Here we describe a new mechanism by which foot-and-mouth disease virus (FMDV) can become resistant to ribavirin. Amino acid changes in the viral polymerase, selected by ribavirin, are able to modify the types of mutations produced in the presence of ribavirin. P44S but not P169S was detected in a 70% proportion in R-Ap35, as evidenced by analysis of both the consensus sequences and their corresponding mutant spectra. These results suggest that the three substitutions in 3D were selected sequentially during replication in the presence of increasing concentrations of R: first M296I, then P44S and finally P169S. To identify possible structural modifications of the viral polymerase associated with the important alterations of the mutational spectrum in progeny RNA, and to investigate how these modifications can affect RNA binding and polymerase activity, the different mutant 3Ds were incubated with the heteropolymeric sym/sub-U RNA of sequence 5′GCAUGGGCCC3′, crystallized, and analyzed by X-ray diffraction.

Two different crystal forms were obtained; the single mutants 3D(P44S) and 3D(P169S) incubated with sym/sub-U RNA crystallized in the tetragonal P42212 space group. The RNA molecule appeared mostly disordered in the two structures. The X-ray structures were determined to 2.2 Å and 2.6 Å resolution for 3D(P44S) and 3D(P169S), respectively, and to 2.6 Å and 2.5 Å for 3D(P44S, M296I) and 3D(SSI), respectively. Subtle domain movements, in particular a ∼1° rotation of the thumb domains relative to the fingers, were observed between the unbound, tetragonal, and the RNA-bound, trigonal structures when the individual domains were superimposed. As a consequence of this rotation, the active site appeared more closed in the unbound state. Thus, the changes observed seem to be a consequence of either RNA-binding, or of the different packing constraints in the tetragonal and trigonal space groups or both, but they do not seem to be related to the presence of substitutions P44S or P169S. Finally, no significant structural changes were observed associated with substitution P169S. Finally, P169 is a non-conserved residue located in motif F of 3D that has been implicated in the recognition of the triphosphate moiety of the incoming nucleotide. P169 is close to 3D residues that directly contact with either the triphosphate or ribose moieties of the incoming nucleotide. However, we can not exclude that a change at this position could also affect the recognition of an incoming nucleotide, modulating its incorporation rate, and thus altering the replication fidelity or replicative fitness.

> GLIVDTRDVEERVHVMRKTKLAPTVAHGVFNPEFGPAALSNKDPRLNEGVVLDEVIFSKHKGDTKMSAEDKALFRRCAADYASRLHSVLGTANAPLSIYEAIKGVDGLDAMEPDTAPGLPWALQGKRRGALIDFENGTVGPEVEAALKLMEKREYKFACQTFLKDEIRSMEKVRAGKTRIVDVLPVEHILYTRMMIGRFCAQMHSNNGPQIGSAVGCNPDVDWQRFGTHFAQYRNVWDVDYSAFDANHCSDAMNIMFEEVFRTEFGFHPNAEWILKTLVNTEHAYENKRITVEGGMPSGCSATSIINTILNNIYVLYALRRHYEGVELDTYTMISYGDDIVVASDYDLDFEALKPHFKSLGQTITPADKSDKGFVLGHSITDVTFLKRHFHMDYGTGFYKPVMASKTLEAILSFARRGTIQEKLISVAGLAVHSGPDEYRRLFEPFQGLFEIPSYRSLYLRWVNAVCGDAAALAHH>[3x]VNFEEVRELVPQKYPFLFIDKVIELQKESRIVCLKNISGNEP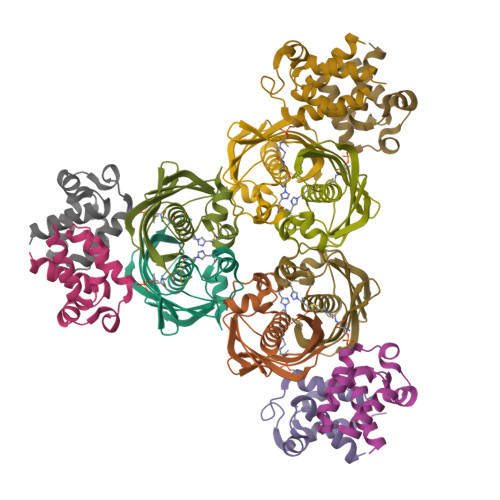FFAGHFPDFAIMPGVLIVEALAQASIILFKKSFSTEQHKDKVFLLASANVRFSKPVFPGDQLILEIDIEKVISSAAIVKGVAKVGDKVVTKATLSFGVANKD;>PVENLEKEITAIVAEVTELDENEIWEKRDADFFKDLEIDSLLALEILALIEKKFKVQIPEEKLVDITSLNATIEMTRSTLEGK[3x]N-{[(1R,2R)-2-(3-fluorophenyl)cyclopropyl]methyl}-2-[2-(1H-imidazol-1-yl)pyrimidin-4-yl]ethanamine 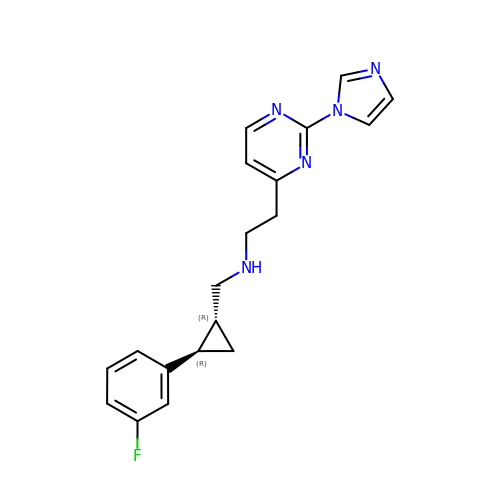| C19 H20 F N5 | GLFSJKKKONEYJI-YJBOKZPZSA-N> MSEFRIHHDVNELLSLLRVHGGDGAEVYIDLLQKNRTPYVTTTVSAHSAKVKIAEFSRTPEDFLKKYDELKSKNTRNLDPLVYLLSKLTEDKETLQYLQQNAKERAELAAAAVGSSTTSINVPAAASKISMQELEELRKQLGSVATGSTLQQSLELKRKMLRDKQNKKNSGQHLPIFPAWVYERPALIGDFLIGAGISTDTALPIVLLRWNLALSPRLKCSGVISAHCNLHLPGTLPLASQESAVVEDLLYVLVGVDGRYVSAQPLAGRQSRTFLVDPNLDLSIRELVHRILPVAASYSAVTRFIEEKSSFEYGQVNHALAAAMRTLVKEHLILVSQLEQLHRQGLLSLQKLWFYIQPAMRTMDILASLATSVDKGECLGGSTLSLLHDRSFSYTGDSQAQELCLYLTKAASAPYFEVLEKWIYRGIIHDPYSEFMVEEHELRKERIQEDYNDKYWDQRYTIVQQQIPSFLQKMADKILSTGKYLNVVRECGHDVTCPVAKEIIYTLKERAYVEQIEKAFNYASKVLLDFLMEEKELVAHLRSIKRYFLMDQGDFFVHFMDLAEEELRKPVEDITPPRLEALLELALRMSTANTDPFKDDLKIDLMPHDLITQLLRVLAIETKQEKAMAHADPTELALSGLEAFSFDYIVKWPLSLIINRKALTRYQMLFRHMFYCKHVERQLCSVWISNKTAKQHSLHSAQWFAGAFTLRQRMLNFVQNIQYYMMFEVMEPTWHILEKNLKSASNIDDVLGHHTGFLDTCL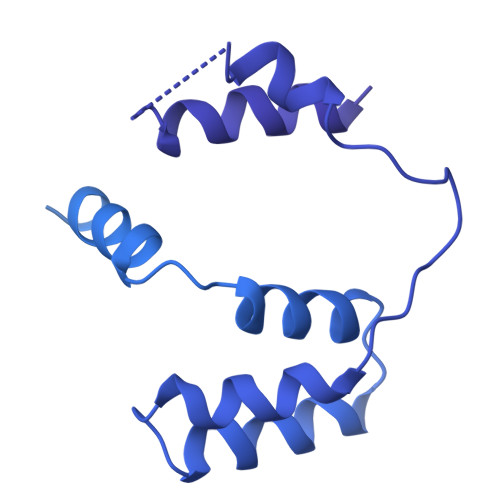KDCMLTNPELLKVFSKLMSVCVMFTNCMQKFTQSMKLDGELGGQTLEHSTVLGLPAGAEERARKELARKHLAEHADTVQLVSGFEATINKFDKNFSAHLLDLLARLSIYSTSDCEHGMASVISRLDFNGFYTERLERLSAERSQKATPQVPVLRGPPAPAPRVAVTAQ> GPDSMEEVVVPEEPPKLVSALATYVQQERLCTMFLSIANKLLPLKPHACHLKRIRRSSATRVATAPMDGFAGG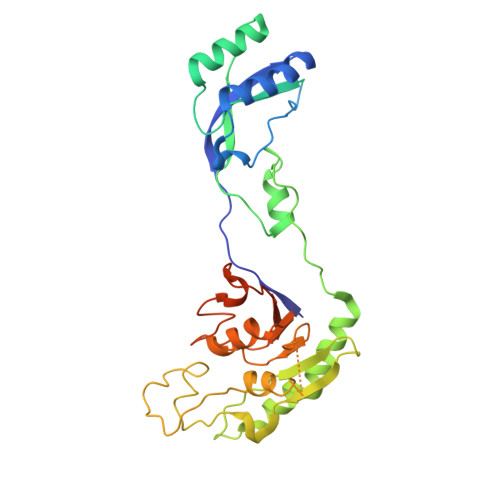VICDKRDSSVATSTISDGCERNSAALGTPAAEKSHVLELLLSVGGPVDSSALKELESAADTTVAVHRVWVPDRAPRSSAEEWTKWCQIWPFATPKPRVPTQLSECEVGSIQRIFRTVVMPLAKRLRTDETLGIAAVLVDPSDGYRVLVSSGEEHALKRGNSAACLGYVSNSGCRKSNRVVLDHPVTFVLKEVTRKQCKDREVEGDASYLANGMDMFVSHEPCVMCSMALVHSRVRRVFYCFPNPVHGGLGSTVSIHAIQELNHHFRVFRCDSRWLSDPEGVSSDHDNPYWEDLTVP> MADEIAKAQVARPGGDTIFGKIIRKEIPAKIIFEDDQCLAFHDISPQAPTHFLVIPKKHISQISAAEDADESLLGHLMIVGKKAAAD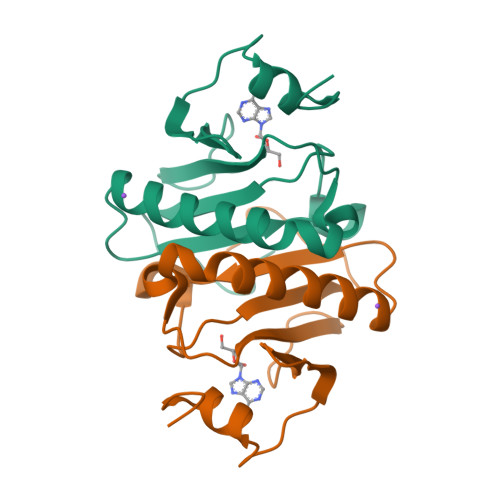LGLKKGYRMVVNEGSDGGQSVYHVHLHVLGGRQMNWPPG4-amino-2-[(3S)-3-(propanoylamino)pyrrolidin-1-yl]pyrimidine-5-carboxamide | C12 H18 N6 O2 | 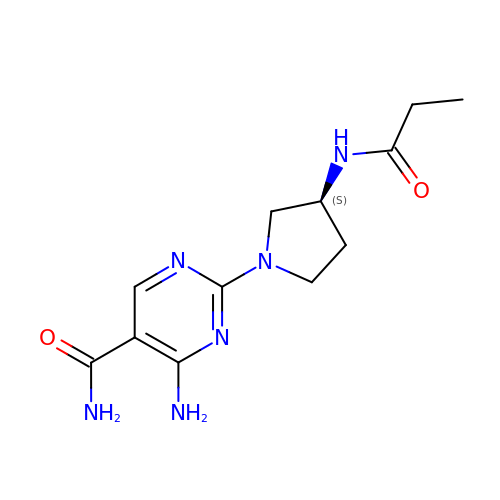RFNYKYSEMVFRHS-ZETCQYMHSA-N IpaH9.8 is one of the most well-studied members of the IpaH family and is secreted by Shigella flexneri during infection. IpaH proteins function as E3 ligases and subvert the host UPS pathway to suppress the host inflammasome and innate immune responses. Recently, it has been reported that IpaH9.8 targets human guanylate-binding protein 1 (hGBP1) for ubiquitination and degradation in order to suppress host defense in cells. In this study, we illuminated the key role of the LRR domain in autoinhibition of IpaH9.8 and revealed that IpaH9.8 can be activated by its LRR domain through substrate binding.

The near full-length structure of IpaH9.8 (truncated the N-terminal T3SS signal sequence) was determined by crystallization and X-ray diffraction at a 2.75 Å resolution. The crystals belonged to a space group I222 with one copy of IpaH9.8 in each asymmetric unit. The final refined model of IpaH9.8 consisted of Thr22–Asp244 within the LRR domain, and Ala255–Ser536 within the NEL domain. The LRR domain of IpaH9.8 adopted an expected solenoid-like structure consisting of eight LRR motifs, with both the N-terminus and C-terminus capped by two helices (right). The NEL domain of IpaH9.8 is an all helical-fold structure, consisting of three subdomains: N-subdomain (from α5 to α8), M-subdomain (from α9 to α13), and C-subdomain (from α14 to α17) (left). In our structure, the α8 and α9 in the NEL domain of the IpaH9.8 (termed IpaH9.8NEL-FL) showed a “helix-loop-helix” fold, with the loop region between α8 and α9 being flexible and not observable in electron density map. The autoinhibition mode of IpaH9.8NEL-FL is similar to IpaH3 in mode 2. Structural analysis revealed that Phe395 in the NEL domain makes hydrophobic contact with Ile196 in LRR-CT, which might be important for IpaH9.8 autoinhibition. Further structural analysis revealed that six hydrophobic residues (Ile196, Leu201, Ile211, Leu216, Leu224, and Ile238) located in LRR-CT constitute a hydrophobic cluster. In addition, this hydrophobic cluster forms a hydrophobic pocket in which the Phe395 of NEL could be confined.

> DPTYADYFSAWDKWEKQALPGEERDEAVSRLKECLINNSDELRLDRLNLSSLPDNLPAQITLLNVSYNQLTNLPELPVTLKKLYSASNKLSELPVLPPALESLQVQHNELENLPALPDSLLTMNISYNEIVSLPSLPQALKNLRATRNFLTELPAFSEGNNPVVREYFFDRNQISHIPESILNLRNECSIHISDNPLSSHALQALQRLTSSPDYHGPRIYFSMSDGQQNTLHRPLADAVTAWFPENKQSDVSQIWHAFEHEEHANTFSAFLDRLSDTVSARNTSGFREQVAAWLEKLSASAELRQQSFAVAADATESCEDRVALTWNNLRKTLLVHQASEGLFDNDTGALLSLGREMFRLEILEDIARDKVRTLHFVDEIEVYLAFQTMLAEKLQLSTAVKEMRFYGVSGVTANDLRTAEAMVRSREENEFTDWFSLWGPWHAVLKRTEADRWAQAEEQKYEMLENEYPQRVADRLKASGLSGDADAEREAGAQVMRETEQQIYRQLTDEVLALRLSENGSQLHHS>UUGCGUCGCGUCGACGAAGUCGC[2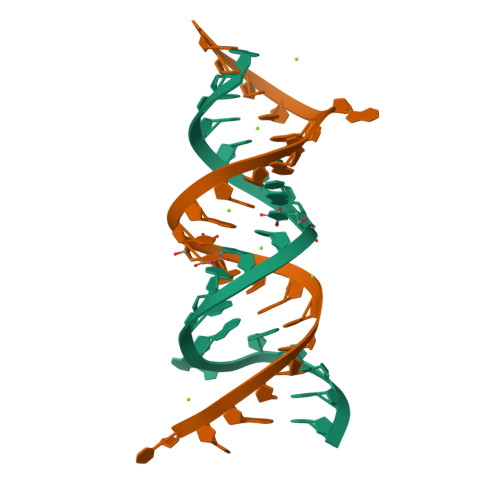x]> MFSESLCILSRRFRYNTKFPALVSYNKLPWEVVNHETPQFHMHVAPHYEQLLTLAASSPVPHIIGSKHIDVPREHRLRLLPGMLYLLDGDTLPGEFTINRVLDPTALQYYGRLSSQIVTVEAVRMLVPDDLRLLCNCITFKGPLHLPVAPYA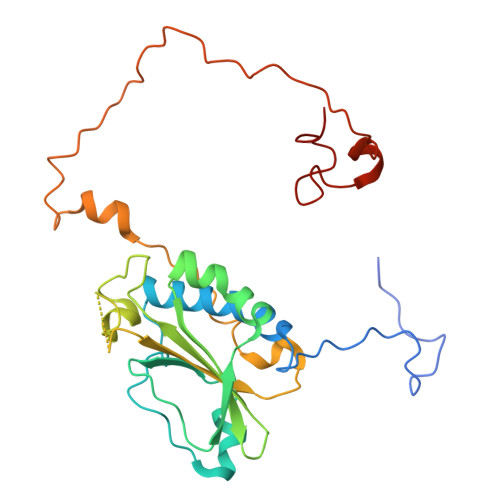SLASLRGASQGGTTGSETGSNCFTLYHFVRPNRPPKELQLEKYYIHAPCVAPLSEFASNSDERGNWRPRLQAPKRTRRATPLPAYRPPQSYLMGLAERLAVVPGGCFGRRSLMWGHWF>MGHHHHHHMKFGPETIIHGDCIEQMNALPEKSVDLIFADPPYNLQLGGDLLRPDNSKVDAVDDHWDQFESFAAYDKFTREWLKAARRVLKDDGAIWVIGSYHNIFRVGVAVQDLGFWILNDIVWRKSNPMPNFKGTRFANAHETLIWASKSQNAKRYTFNYDALKMANDEVQMRSDWTIPLCTGEERIKGADGQKAHPTQKPEALLYRVILSTTKPGDVILDPFFGVGTTGAAAKRLGRKFIGIEREAEYLEHAKARIAKVVPIAPEDLDVMGSKRAEPRVPFGTIVEAGLLSPGDTLYCSKGTHVAKVRPDGSITVGDLSGSIHKIGALVQSAPACNGWTYWHFKTDAGLAPIDVLRAQVRAGMN[2x]

Genomic DNA adenine methylation within 5’-GANTC-3’ sequences (N = any nucleotide) is an epigenetic mark that controls gene expression in alpha-proteobacteria. Like the mammalian DNA cytosine methyltransferase (MTase) Dnmt12, which is essential for maintenance methylation of hemimethylated CpG dinucleotides at DNA replication forks, the DNA adenine MTase (Dam) in Escherichia coli and cell cycle-regulated DNA MTase (CcrM) in Caulobacter crescentus are responsible for maintenance methylation of GATC or GANTC immediately after replication, respectively. Here, by means of X-ray crystallography, we show that a CcrM dimer binds DNA by opening up double stranded DNA at the recognition site, a DNA recognition mechanism that likely contributes to the enzyme’s sequence discrimination. Each molecule comprises an N-terminal MTase domain (residues 1–260) of an 8-stranded β-sheet (β1-β8) with three helices (αA, αB, αC, and αE, αF, αG) located on each side of the sheet, resulting in an open αβα sandwich.

We used an 18-base-pair oligonucleotide (plus a 5’-overhanging cytosine on one strand and a guanine on the other strand) containing a non-centrally located GAATC site for co-crystallization with CcrM. We crystallized the CcrM-DNA complex in the presence of sinefungin (a methyl donor analog) in space group P212121 and determined the structure to the resolution of 2.34 Å. The DNA-bound form of CcrM contains two molecules (A and B). The dimer interface with an area of ~3100 Å2 is mainly mediated by the MTase domains with two active sites (indicated by the binding of sinefungin) facing opposite directions. The MTase domain of molecule A (in cyan) makes most of the contacts to the target strand (in magenta) and catalyzes methyl transfer, while the C-terminal domain of molecule B (in green) is solely responsible for the binding of the non-target strand (in yellow). The CcrM-bound DNA molecule undergoes dramatic distortions at the 5-bp recognition site while the outer sequences at both ends maintain B-form. Subsequently, four out of the five base pairs within the recognition sequence are disrupted (A2:T2 to C5:G5), with the four bases of the target strand (A2 to C5) being repositioned into new locations and being completely out-of-stacking with neighboring bases. In molecule A, the 30-residue Loop-2B approaches DNA from the major groove with the tip of the loop, Pro45, wedging in-between the two thymine bases T2 and T3, causing a kink in the non-target strand and displacing thymine T2 to the border of the double helix. In accordance with the most common mechanism for guanine recognition, Arg44 forms bidentate hydrogen bonds with the O6 and N7 atoms of the G1 base.>SAPVSIWSRVVQFGTGWGFWVSGHVFITAKHVAPPKGTEIFGRKPGDFTVTSSGDFLKYYFTSA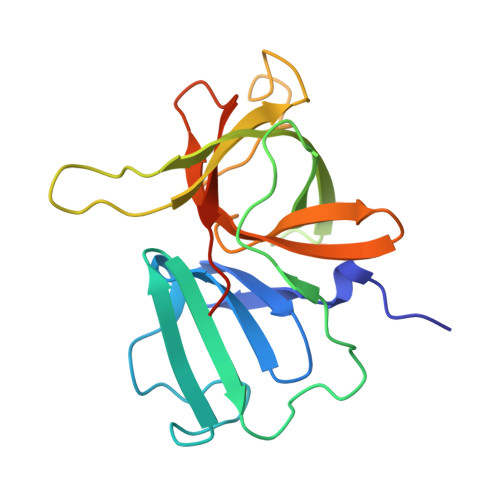VRPDIPAMVLENGCQEGVVASVLVKRASGEMLALAVRMGSQAAIKIGSAVVHGQTGMLLTGSNAKAQDLGTIPGDAGCPYVYKKGNTWVVIGVHVAATRSGNTVIAATHGEPTLEALEFQG[4x];> LEFQG> GREEAPNAEADILSCRLPGVVMTTSPIITNNSINIFVGPGTDISSLAPEFTLTPGATIDPPSGTARDFHSPQQYTVTAADGFWKKKYTVSVIDTELATIYNFEDTLGGQKYYIFVEREGEKVVMEWASGNAGYAMTGVPKTADDYPTFQFANGKTGKCLSLVTRSTGFFGSIMGMPIAAGNLFIGSFDVGNAMSNPLKATKFGLPFRHIPTYLAGYYKYKAGDQFTEGGKPVSGKRDICDIYAIMYETSESVPTLDGTNAFTSPNLVSIARIDDAKETDEWTYFKLPFHMLSGKYIDKEKLTAGKYNVAIVFTSSLEGDHFNGAIGSTLLIDEVELIYRSED

BT2081 from Bacteroides thetaiotaomicron (GenBank accession code NP_810994.1) is a member of a novel protein family consisting of over 160 members, most of which are found in the different classes of Bacteroidetes. Genome-context analysis lends support to the involvement of this family in carbohydrate metabolism, which plays a key role in B. thetaiotaomicron as a predominant bacterial symbiont in the human distal gut microbiome. BT2081 consists of an N-terminal domain, which adopts a β-sandwich immunoglobulin-like fold, and a larger C-terminal domain with a β-sandwich jelly-roll fold. The C-terminal β-jelly-roll domain contains a potential carbohydrate-binding site that is highly conserved among BT2081 homologs and is situated in the same location as the carbohydrate-binding sites that are found in structurally similar glycoside hydrolases (GHs).

The crystal structure of BT2081 was determined to 2.05 Å resolution using the SAD method. The final model includes one BT2081 molecule (residues 21–360), two calcium ions, two sodium ions, two cacodylate anions, two acetate anions, 19 polyethylene glycol molecules and 251 water molecules in the asymmetric unit. Crystallographic packing, as well as PISA analyses of BT2081, suggest that a monomer is likely to be the biologically relevant form of the protein, which is consistent with results from analytical size-exclusion chromatography (anSEC). A calcium ion is present in the N-terminal domain on the surface near the start of the domain. Unlike those proteins, however, the calcium in the BT2081 N-terminal domain is quite solvent-exposed and, as three of the six ligands are solvent molecules and another is a crystallographically related molecule, this bound calcium ion is most likely to be an artifact of crystallization. Another shared feature is a conserved calcium-binding site on the convex surface of the β-jelly roll. In BT2081, this calcium is octahedrally coordinated by a water molecule, the carbonyl O atoms of Asn120, Thr174 and Lys176 and the carboxylate O atoms of Glu122 and Asp351. As a consequence of these extended loop regions, a significant distinction between BT2081 and its structural counterparts is the presence of a deep solvent-accessible pocket in BT2081 formed by highly conserved residues from the concave surface of the β-jelly-roll core and five of the loop regions extending from this core. Similar to the carbohydrate-binding sites found in type B CBMs, the putative binding pocket of BT2081 contains several highly con­served aromatic residues arranged in such a way that they form a twisted platform to which a potential polysaccharide could bind. Of these residues, Asp259 and Asp338 at the bend of the pocket are particularly interesting candidates for performing catalytic roles because they are positioned opposite each other in the pocket, with their carboxylate O atoms being sufficiently far apart (∼7.5 Å) to accommodate a carbohydrate substrate.Typically, TCSs consist of a sensor histidine kinase (HK) and a response regulator (RR). Prototypical HKs are membrane-bound dimers comprising a sensor domain that detects their cognate stimuli, a catalytic ATP binding domain (CA) that binds ATP and, upon signal detection, autophosphorylates a conserved histidine in the dimerization, and a histidine phosphotransfer domain (DHp). The ATP-binding pocket of HKs adopts the Bergerat fold, an α/β sandwich characterized by four conserved regions (the N-box, the G1-box, the G2-box, and the G3-box) and the highly variable ATP-lid. The Bergerat fold has been observed in the ATP-binding domain of the GHKL protein superfamily, which includes DNA gyrases, the molecular chaperone Hsp90, bacterial HKs, and the MutL mismatch repair enzyme.

Our attempts to co-crystallize the DPP derivative with the CA domain of CheA from T. maritima, a class II HK for which robust crystallization protocols have been established, failed. However, we successfully obtained the X-ray crystal structure of the resorcinol fragment bound to CheA-CA with a resolution of 2.1 Å. The overall structure showed a solvent-accessible binding pocket where the resorcinol was observed making contact with the conserved aspartate (Asp449): the one hydroxyl from the resorcinol is in the proximity of the conserved aspartate (Asp449) and the ordered water molecule W1, while the other hydroxyl of the resorcinol forms water-bridged contacts with the backbone carbonyl a leucine residue (Leu406; Val386 in PhoQ E. coli). The binding mode of the resorcinol resembles the predicted binding mode of DPP-5 and is nearly identical to the interaction formed by the DPP CCT018159 with Hsp90α. The crystal binding mode of the resorcinol fragment supports the hypothesis that resorcinol-containing DPP compounds are likely to retain the binding mode observed in Hsp90. Docking studies indicate that the substitution pattern on ring A influences the binding mode, with the resorcinol-based derivatives likely to adopt a binding mode analogous to the crystal-bound complex of CCT018159-Hsp90α, an observation also supported by the X-ray crystal structure of resorcinol in complex with the HK CheA. The CheA-CA domain was crystallized by the sitting-drop vapor-diffusion method at 21°C using 0.4 µL of 25 mg/mL CheA-CA protein mixed with 0.4 µL of reservoir solution containing 30% (wt/vol) PEG 8000, 0.6 M ammonium acetate, 0.065 M sodium acetate pH 4.5. Monoclinic crystals appeared within 24 hours, and 0.2 µL of 20 mM resorcinol solution (Enamine, Frankfurt, Germany) was added to the crystallization drops. The part of the lid loop corresponding to residues 492–505 could not be built owing to the absence of the corresponding electron density in the area.

>GSHMVPISFVFNRFPRMVRDLAKKMNKEVNFIMRGEDTELDRTFVEEIGEPLLHLLRNAIDHGIEPKEERIAKGKPPIGTLILSARHEGNNVVIEVEDDGRGIDKEKIIRKAIEKGLIDESKAATLSDQEILNFLFVPGFSTKEKVSEVSGRGVGMDVVKNVVESLNGSISIESEKDKGTKVTIRLPLT[2x]> XKGIVTGAVSD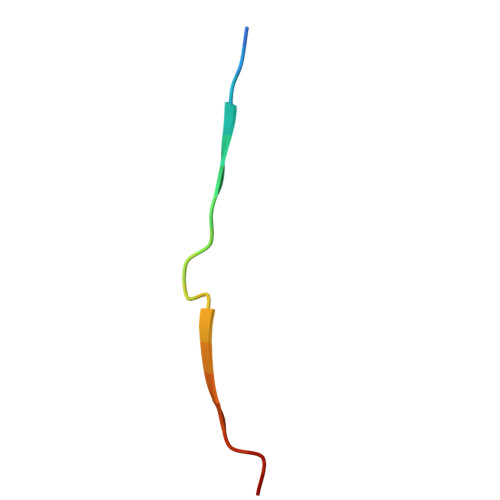HTTVEDTKX>[2x]MELRKGLEDIAIKETSITYIDGELGRLYYRGYSIFDLASFSNFEEVAYLLWYGKLPTRHELDDFKSRLAEERSISEDISTFVKRTAKFGNPMDILRTTVSMMGLEDRSEGDLIGKAIKMTAKIPTIISLIQRTRRNQEFVEPDPSLSHSENFLYMIRGERPSPSDTRVLDVSLMLHMDHEMNASTMACLVVASTLSDIYSSVVAGISALKGPLHGGANSEALKQFMEIETPDNVEKYVMNKLSSGQRLMGFGHRIYKTMDPRAKILKEYANQLSKNEEIKRLFEIANRVEEIGIKILGKRGIYPNVDFYSGLVFYAMGFDPDLFPTIFASARVIGWTAHVDEYLKDNKLIRPKAIYVGDLGKRYVPIEERLEHHHHHH

Citrate synthase of M. sedula (MsCS) catalyzes the first step of the incomplete TCA/glyoxylate cycle in this strain. CSs (EC 2.3.3.1) catalyze conversion of oxaloacetate and acetyl-CoA into citrate and coenzyme A and are well-conserved enzymes in most organisms. The findings reveal that the protein functions as a dimer, similar to other Type-I CSs. The monomeric structure of MsCS consists of seventeen α-helices (α1-α17) and four β-strands (β1-β2), with distinct large domain and small domains.

In order to reveal oxaloacetate binding mode of MsCS, high concentration of oxaloacetate was added to the purified MsCS protein at the crystallization step. MsCS crystals in complex with oxaloacetate were successfully obtained, and we determined its crystal structure at 2.0 Å at pH 7.24 condition. The structural examination revealed two MsCS molecules and two glycerol molecules in the asymmetric unit. The oxaloacetate binding pocket is almost identical with the citrate binding pocket and is formed by two α-helices (α13 and α16) and three loop regions (α8-α9, α10-α11, and α12-α13). In the large domain, Asn182 interacts with the C2 and C3 carboxyl-groups and Arg332 stabilizes the C3 carboxyl-group of oxaloacetate via a salt bridge. In addition, His253 from the small domain interacts with the C3 carbonyl-group and Arg262 is associated with the stabilization of C3 carbonyl- and carboxyl-groups of oxaloacetate through hydrogen bonds. Interestingly, Asn182 is not conserved in other CS proteins, and some other CS structures contain Pro at the corresponding position, indicating that stabilization mode of oxaloacetate might be somewhat different among CSs. However, detailed comparison of the structure of MsCS in complex with oxaloacetate with that in complex with citrate revealed that the conformation of these structures were somewhat different from each other. While Arg351 interacts with the citrate product, this residue does not interact with the oxaloacetate substrate, but rather rotates away from the compound.>[2x]MAHHHHHHVGTFENITAAPADPILGLADLFRADERPGKINLGIGAYIDETGKFPVLTSVKKAEQYL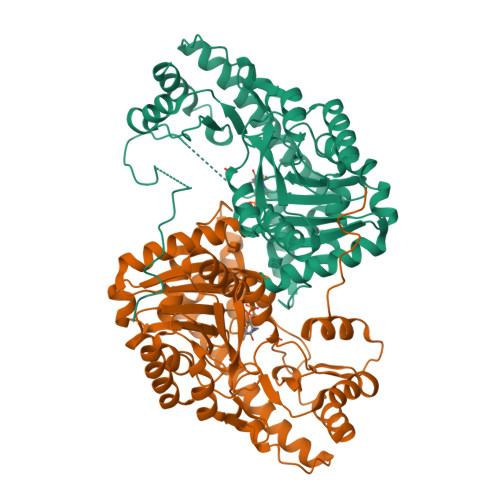LENETTKSYLGIDGIPEFGRCTQELLFGKGSALINDKRARTAQTPGGTGALRVAADFLAKNTSVKRVWVSNPSWPNHKSVFNSAGLEVREYAYYDAENHTLDFDALINSLNEAQAGDVVLFHGCCHNPTGIDPTLEQWQTLAQLSVEKGWLPLFDFAYQGFARGLEEDAEGLRAFAAMHKELIVASSYSKNFGLYNERVGACTLVAADSETVDRAFSQMKAAIRANYSNPPAHGASVVATILSNDALRAIWEQELTDMRQRIQRMRQLFVNTLQEKGANRDFSFIIKQNGMFSFSGLTKEQVLRLREEFGVYAVASGRVNVAGMTPDNMAPLCEAIVAVL>MGSSHHHHHSSGENLYFQMMDGVEGGTAMYGGLETVQYVRTHHQHLCRENQCTSALVK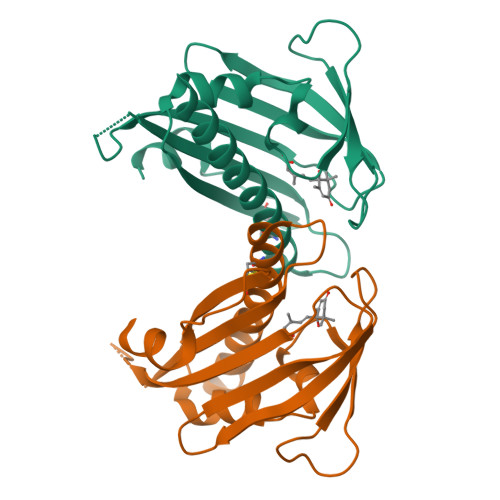HIKAPLHLVWSLVRRFDQPQKYKPFVSRCTVIGDPEIGSLREVNVKSGLPATTSTERLELLDDEEHILGIKIIGGDHRLKNYSSILTVHPEIIEGRAGTMVIESFVVDVPQGNTKDETCYFVEALIRCNLKSLADVSERLASQDITQ[2x]> MGSSHHHHHHSSGRENLYFQGMRKFIIVKNVKVDGINAKSSDITVGMPPATTFCGLGETMSIKTGIVVKAVSYGSVKFEVRGSRFNTSVTKFAWQD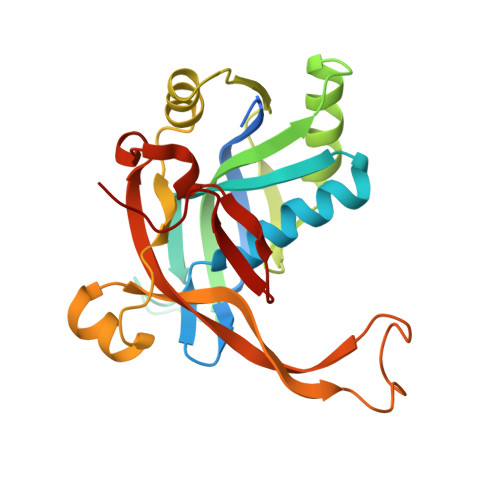RGNGGKANNNSPIQPKPLADGVFTLCFEVEWEDCAEVLVDKVTNFINTARIAGGTIASFNKPFVKVAKDAEELASVKNAMMPCYVVVDCGVEVNIFEDAVNRKLQPMVNGYKKLEKIVDNKHMRDKFTPAYLATPTYTMIGYKMVSNVDNFDQALWQYGENTKVKTIGGIYND Phycobilisomes (PBS) are antenna megacomplexes that transfer energy to photosystems II and I in thylakoids. Here we show the cryo-EM structure at a global resolution of 2.9 Å of the 5.9-MDa PBS from Anthocerotibacter panamensis (hereafter A. panamensis), a recently discovered Gloeobacterial species that diverged from Gloeobacter spp. around 1.4 billion years ago. The A. panamensis PBS features a configuration comprising two herein characterized linkers and presents a paddle-shaped morphology. The two-fold symmetric PBS contains twelve APC hexamers assembled as a heptacylindrical core surrounded by twelve PC hexamers, with approximate dimensions of 273 Å (width), 500 Å (height), and 129 Å (thickness).

The heptacylindrical core in A. panamensis has two distinct complexes—the bottom pentacylindrical and the top bicylindrical subcomplexes—each with a different combination of Apc protein components. Instead, ApcA2, ApcB2, ApcB3, ApcC2, and ApcE form the bottom pentacylindrical core, and these five proteins are phylogenetically close to their homologs in crown Cyanobacteria. However, both ApcD and ApcF are absent in the A. panamensis PBS. Although ApcB3 only exists as a single copy like ApcF of hemidiscoidal PBS in each bottom core cylinder, ApcB2 (β3) is found at the positions occupied by ApcF in other pentacylindrical core structures and is likely the functional equivalent to ApcF that occurs in crown Cyanobacteria. Additionally, the position of ApcD is occupied by an ApcA2 (α1) subunit in the paddle-shaped PBS. The EET from the top core cylinders to the pentacylindrical core is also efficient, given that the bilin distance between D’ and B’ cylinders is similar to the ones within the pentacylindrical core. Although the positions of A'2βApcB2 and A'1αApcA2 are similar to the bilins in ApcF and ApcD in other structures, it requires further validation if they are functional equivalents to ApcD and ApcF because ApcA2 and ApcB2, unlike ApcD and ApcF, are not single-copy subunits in an APC cylinder. The linker proteins were suggested to provide microenvironments for the bilins and are key bridges in energy transfer in PBS, namely the linker-guided pathway. Both linker-guided and non-linker-guided pathways are identified in the pentacylindrical core. The final overall resolution of APC core complexes ranged from 2.38 Å to 2.73 Å, allowing the assignment of all APC subunits precisely based on the corresponding amino acid sequences.

> MPIKGTSGSNIARPRFYNTVMVETIEGANAEERYFNPGELSSMAGFFNDAQRRLAIVQILTTNAEAIVSRAAGRIFTGGSPMAFSVQQANRQKDAEKERVSARVVQAESEQPIGNEVVIEDKGGFLERLKSFFSYGGAEVETPGFRPIPIAVYGPERMQKSLRDLDWFLRYVNYSLVAGDSNMILLNCLGLREILEKACSIDATIVAVQEMRRAATGYLKSNDDKELVGSYFDVIIRSLNADKSDTPADVVRPSSPDRAGLVLPAIYALAGQSRPAFKMSRTLTSAEKERVVRAAYRQVFERDILAYGQSISYLDSKVKNGEISVKEFIRLLGKSELYRKQFFEPFINSRVLELAFKHFLGRAPESRTEVQNYYSIVAAQGLGGLVDALVDGEEYGRIFGEDTVPFIRDLGQEAQPSWNWGAAYSLYNYAAPRRKVPQFITLYADYVKPLPNQHPYGSGNDPLEIQFGAIFKSETKAPSARPAPIGKDVQRILIRSGNPITNERGNPAGGISDKTSLSPQIFKLTQDNRRIRGKSGKGSLITNAGAGSVEVNVQAVIRAAYQQVFGRQLYEGQHLSVSEIKLENGEISVKEFVRDLATSEIFRKLYWQNFYVCKSIEYIHRRLLGRPTYGRDETNRYYDLAFKKGFAGVVNAILDTMEYAEVFGDDVVPYERYVTPAGLNLRKLRAGTVPTLPSFEETPKFIEKGTAPDRALPQIRSAINQGVSKKRDQRKIFSTVGIQTSLASRTEFDALIRAAYRQVFERDMDSYRITEVFSVLETKLRNREITTKEFIQALASSDLYRKQFFEPYPPTKNVELSLKHLLGRATKDQAELRKYNQIIATQGFKPFINAILDSKEYGEVFGDGTVPYNRYPTLPAANFPNTEILYNQLTKQSAEVVVPSFKPVTSPRGMDMSQTPLMLQAMGDIAEAEQEVALQKPLFIQKGKALRGAEGDPYTIGTRRSPKPIFWVPQGGTNPTEFQNVIRAAYRQVFERDVPDYQRLSYPESRLKNGEISMREFIRQLAESDLYRKQFYEPYPNTKVIELLTKHFLGRAPQDQAEIQRYNRILAGKGLKVAIEEVLNSDEYTQLFGEDVVPFKRYPTLPTGTYLASVATNDEMIQQSGSSYSPSYAGYSYPFS;>[23x]MSVVTKAIVSADAEARYLSPGELDRIRGFVSSGERRLRVAQTLTESRERIIKQAGDQLFQKRPDLVSPGGNAYGAERTASCLRDLDYYLRLVTFGIVAGDVTPIEEIGVIGVKEMYRNLEVPLPGMVEAVKAMKSVATGLLSGDDSAEVGYYFDYLAGALA;> MQDVIGKVIAEYDTKGKYLDAAALDLLRSYFDSGDLRLKAAQAITANAEVIVRAASAKALHYTPVTKPGGNMYYARRYASCIRDLDYFLRYATYAMLADNTTLLDEYVLKGLTETYRALGVPLDISVRAINALKEVVAGQVGPKAGQEMAKYFDHLAKGLG;>[23x]MQDAITSVINTYDVQGKYFDTSAFDKLKAYYATGELRVRAAGTISANAATIIKEASAKLFSNQPDLVRPGGNAYTTRRYAACVRDMDYFLRYATYAMLAGDTSILDERVLNGLKETYNSLGVPISSTVQGIQAMKEVTGSLVGSGAAKEMGVYFDYLSSGLS;>MTRLFKVTALIPSYKKVRGGRELQNTYFTKLVEYDRWFAEQQRIQKQGGKILSVKMVAGKPGLNTGVL[4x]> GGACAGCCTGTACGGACATCA;> CC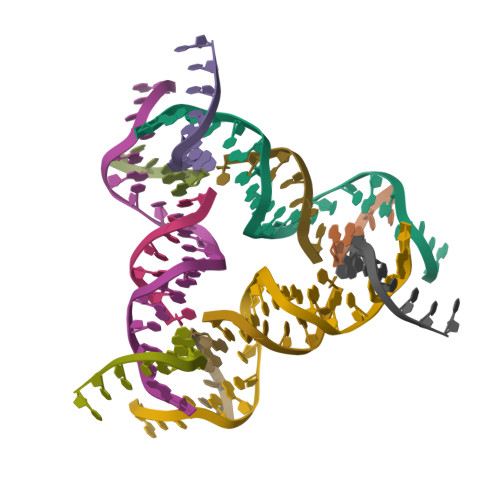GTACA;> GGCTG;> CTCTGATGT>[2x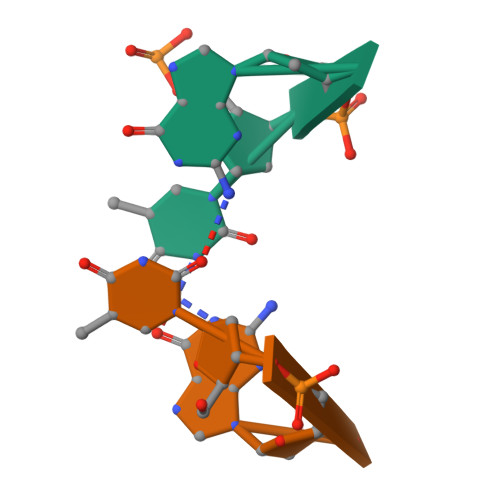]TGTG> NAPTAVKKDAPSEVTKAASSENASSAKLSVPERQKLAQQSAGKVLTLLDLSEVQLDGAATLVLTFSIPLDPDQDFSRVIHVVDKKSGKVDGAWELSDNLKELRLRHLEPKRDLIVTIGKEVKALNNATFSKDYEKTITTRDIQPSVGFASRGSLLPGKVVEGLPVMALNVNNVDVNFFRVKPESLPAFISQWEYRNPLANWQSDKLLQMADLVYTGRFDLNPARNTREKLLLPLGDIKPLQQAGVYLAVMNQAGRYDYSNPATLFTLSDIGVSAHRYHNRLDIFTQSLENGAAQQGIEVSLLNEKGQTLTQATSDAQGHVQLENDKNAALLLARKDGQTTLLDLKLPALDLAEFNIAGAPGYSKQFFMFGPRDLYRPGETVILNGLLRDADGKALPNQPIKLDVIKPDGQVLRSVVSQPENGLYHFTWPLDSNAATGMWHIRANTGDNQYRMWDFHVEDFMPERMALNLTGEKTPLTPKDEVKFSVVGYYLYGAPANGNTLQGQLFLRPLREAVSALPGFEFGDIAAENLSRTLDEVQLTLDDKGRGEVSTESQWKETHSPLQVIFQGSLLESGGRPVTRRAERAIWPADALPGIRPQFASKSVYDYRTDSTVKQPIVDEGSNAAFDIVYSDAQGVKKAVSGLQVRLIRERRDYYWNWSEDEGWQSQFDQKDLIENEQTLDLKADETGKVSFPVEWGAYRLEVKAPNEAVSSVRFWAGYSWQDNSDGSGAVRPDRVTLKLDKASYRPGDTIKLHIAAPTAGKGYAMVESSEGPLWWQEIDVRAQGLDLTIPVDKTWNRHDLYLSTLVVRPGDKSRSATPKRAVGVLHLPLGDENRRLDLALETPAKMRPNQPLTVKIKASTKNGEKPKQVNVLVSAVDSGVLNITDYVTPDPWQAFFGQKRYGADIYDIYGQVIEGQGRLAALRFGGDGDELKRGGKPPVNHVNIVVQQALPVTLNEQGEGSVTLPIGDFNGELRVMAQAWTADDFGSNESKVIVAAPVIAELNMPRFMASGDTSRLTLDITNLTDKPQKLNVALTASGLLELVSDSPAAVELAPGVRTTLFIPVRALPGYGDGEIQATISGLALPGETVADQHKQWKIGVRPAFPAQTVNYGTALQPGETWAIPADGLQNFSPVTLEGQLLLSGKPPLNIARYIKELKAYPYGCLEQTASGLFPSLYTNAAQLQALGIKGDSDEKRRASVDIGISRLLQMQRDNGGFALWDKNGDEEYWLTAYVMDFLVRAGEQGYSVPTDAINRGNERLLRYLQDPGMMSIPYADNLKASKFAVQSYAALVLARQQ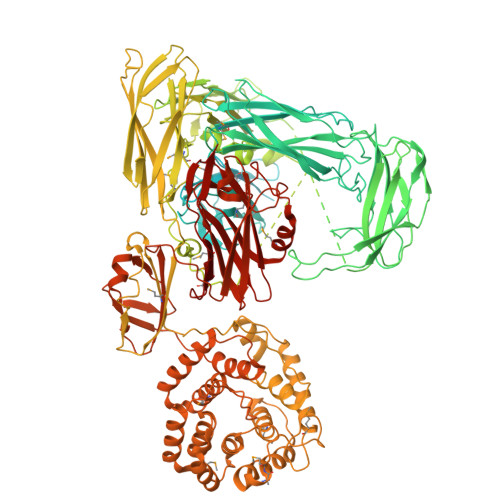KAPLGALREIWEHRADAASGLPLLQLGVALKTMGDATRGEEAIALALKTPRNSDERIWLGDYGSSLRDNALMLSLLEENKLLPDEQYTLLNTLSQQAFGERWLSTQESNALFLAARTIQDLPGKWQAQTSFSAEQLTGEKAQNSNLNSDQLVTLQVSNSGDQPLWLRMDASGYPQSAPLPANNVLQIERHILGTDGKSKSLDSLRSGDLVLVWLQVKASNSVPDALVVDLLPAGLELENQNLANGSASLEQSGGEVQNLLNQMQQANIKHIEFRDDRFVAAVAVDEYQPVTLVYLARAVTPGTYQVPQPMVESMYVPQWRATGAAEDLLIVRPLEHHHHHH Inner kinetochore proteins, particularly members of the Ctf19c, constitute the foundation of the kinetochore; they both recognize Cse4/CENP-A and recruit microtubule-interacting outer kinetochore proteins. The Ctf3c namesake, Ctf3, is a 733 amino-acid residue protein predicted to consist almost entirely of HEAT repeats (Huntingin, elongation factor 3 (EF3), protein phosphatase 2A (PP2A), and yeast kinase TOR1 repeats). Ctf3 associates with a coiled-coil dimer of Mcm16 and Mcm22 (Mcm16/22).

We now present a cryo-EM structure of the yeast Ctf3c, which resolves the overall organization of the complex, shows how Ctf3 binds Mcm16/22, and clarifies Ctf3c recruitment to the larger Ctf19c. The final map shows side-chain density throughout the particle, enabling modeling at near-atomic resolution. We modeled five Ctf3-C HEAT repeats, which have the overall fold of canonical HEAT arrays. Nearly 120 amino acid residues interrupt an imperfect sixth repeat at the C-terminal end of the modeled peptide chain, making a helical knob. As we saw in the previous Ctf3c model, an Mcm16/22 coiled-coil occupies the cleft formed by the concave surface of the HEAT array. The two main components of the structure, Ctf3-C and Mcm16/22 N, have opposite polarities; the central parts of Mcm16 and Mcm22 form a parallel coiled-coil that begins near the C-terminal end of the modeled Ctf3 polypeptide. The N-terminal parts of Mcm16 and Mcm22, form a set of four interdigitated helices that pack onto the convex side of the C-terminal part of the HEAT array and contact the helical knob. The final model shows that the structure determined here (Ctf3-C-Mcm16/22 N) is essentially the precise complement of the Ctf3-N-Mcm16/22 C crystal structure. Therefore, the Mcm16/22 dimer extends without a major interruption along the Ctf3 HEAT repeats, forming two tightly but flexibly linked structural modules: Ctf3-N-Mcm16/22 C and Ctf3-C-Mcm16/22 N. The new Ctf3c map also enabled unambiguous identification of the Ctf3 residues that contact Iml3 and likely contribute to Ctf3c kinetochore recruitment.

> SNAMTNSSEKQWERIQQLEKEHVEVYRELLITLDRLYLIRKHNHAVILSHTQQRLLEIRHQLQINLEKTALLIRLLEKPDNTNVLFTKLQNLLEESNSLDYELLQSLGAQSSLHKQLIESRAERDELMSKLIELSSKFPKPTIPPDDSDTAGKQVEVEKENETIQELMIALQIHSGYTNISYTI;> SNAMSLILDDIILSLTNANERTPPQALKTTLSLLYEKSKQYGLSSPQLQALVRLLCETSIIDTVTKVYIVENCFLPDGYLTKELLLEIINHLGTPTVFSRYRIQTPPVLQSALCKWLVHVYFLFPVHSEREHNISSSIWLHLWQFSFLQKWITPLVIWQATTPVDVKPWKLSIIKRCAMHPGYRDAPGSATLILQRFQCLVGASSQITESIITINCNRKTLKSHRNLKLDAHFLSILKRILSRAHPANFPADTVQNTIDMYLSEIHQLGADSIYPLRLQSLPEYVPSDSTVSLWDVTSLEQLAQNWPQLHIPNDVDYMMKPSLNSNVLLPRKVMSRDSLKHLYSSIILIKNSRDESSSPYEWCIWQLKRCFAHQIETPQEVIPIIISVSSMDNKLSSRIIQTFCNLKYLKLDELTLKKVCGGILPLWKPELISGTREFFVKFMASIFMWSTRDGHDNNCTFSETCFYVLQMITNWVLDDKLIALGLTLLHDMQSLLTLDKIFNNATSNRFSTMAFISSLDILTQLSKQTKSDYAIQYLIVGPDIMNKVFSSDDPLLLSAACRYLVATKNKLMQYPSTNKFVRMQNQYIMDLTNYLYRNKVLSSKSLFGVSPDFFKQILENLYIPTADFKNAKFFTITGIPALSYICIIILRRLETAENTKIKFTSGIINEETFNNFFRVHHDEIGQHGWIKGVNNIHDLRVKILMHLSNTANPYRDIAAFLFTYLKSLSKYSVQNS;> SNAMDVEKDVLDVYIKNLENQIGNKRYFLKQAQGAIDEITKRSLDTEGKPVNSEVFTELLRKPMFFSERADPIGFSLTSNFLSLRAQSSSEWLSLMNDQSVDQKAMLLLQNNINSDLKELLRKLQHQMTIMDSKKQDHAHIRTRKARNKELWDSLADFLKGYLVPNLDDNDESIDSLTNEVMLLMKRLIEHDLNLTLNDFSSKTIPIYRLLLRANIITVIEGSTNPGTKYIKLIDFNETSLT>MYQAGGTIRSLLDKVAEQEYLLPAIQREFVWRPEQICRLFDSLLQGYPFGTFLFWKIKPENRDSYQFYQFMQHYHERDNYHCENVTQLPEREFIAVLDGQQRITALNIGLRGSFAWKLTGKWWSNDDAFPVRRLHLNLLSKPDLETGSMYDFEFLTDDKASLDASEQYWFRVGRIMEEEEDALIDEVADDARLSSEQRKEARSTLRHLYRTIHDKDKISFYEESDQSLERVLNIFIRMNSGGTTLSYSDLLLSIAVAQWSSLDAREEIHALVDEMNRVGDGFNVSKDLVLKAGLMLSDIGSVGFKVENFNKENMAILEKNWTPIRDALLLSMQLLASFGFNAQNLRATSAILPLAYYLHHRKLTASYLSRVEYAVDRECIRNWLIRSLLKASGIWGSGLDTLLTMLRSDIKQSGDTGFPLAKIEATMQQRGKSLRFDPEEISELAQLDYGNPRTFALLTLLFPGFDFSRHFHVDHIYPKGLFTRNKLAKVGVPAEQLDELIEASNKLPNLQLLEGTINNQKRQKMPHEWYAQQWPDVNARQAHLQSQAITSLPEQLNQFMDFYRERQETLLARIRTALQPASSVETE[2x]

Using a suite of thirty environmentally-isolated coliphages, we demonstrate multi-layered and robust phage protection provided by a plasmid-encoded defence island that expresses both a type I BREX system and the novel GmrSD-family type IV DNA modification-dependent restriction enzyme, BrxU. The BrxU protein contains DUF262 and DUF1524 domains, and shares 13% amino acid sequence identity with the single polypeptide type IV restriction enzyme GmrSD. Here, we have shown that BrxU is a promiscuous enzyme that uses a range of nucleotide and metal co-factors to recognise and cleave DNA that contains any of at least three different modifications, and this activity is dependent on the initial nucleotide-driven dissociation of BrxU dimers, and subsequent nucleotide hydrolysis. Our BrxU structures are the first for the GmrSD family, providing the highest resolution detail for the widespread DUF262 and DUF1524 domains.

Whilst using the first BrxU structure to analyse datasets from a range of BrxU crystals, a second dimeric structure with a differing conformation of BrxU was solved, this time to 2.85 Å. Our models described above for DNA-binding and dimer dissociation rely upon a great deal of flexibility. By aligning the two solved structures, domain movements were visualised within the BrxU dimer. The overall alignment provides an RMSD of 3.85 Å, indicating a poor average superposition. By aligning the lower resolution structure through one C-terminal domain of the higher resolution protomer, (which as independent domains aligned well at 0.58 Å), distinct relative movements of each of the other domains of the lower resolution structure can be observed. In this manner, we can see a 10 Å movement of the protomeric N-terminal domain, and corresponding shifts of 12 and 26 Å for the N-terminal and C-terminal domains of the second protomer, respectively. This level of movement confirms the flexibility of the BrxU dimer, and gives rise to an hypothesis that the 21 Å cleft might widen to accommodate a substrate DNA, with backbone phosphates supported by loops of the DUF1524 domain, as was seen for the observed sulphate and chloride ions. The structures reveal how nucleotide binding is blocked in the dimer form and reveals inherent flexibility that would allow for cycles of dimer separation.>MDIKINDITLGNNSPFVLFGGINVLESLDSTLQTCAHYVEVTRKLGIPYIFKASFDKANRSSIHSYRGVGLEEGLKIFEKVKAEFGIPVITDVHEPHQCQPVAEVCDVIQLPARLAQQTDLVVAMAKTGNVVNIKKPQGLSPSQMKNIVEKFHEAGNGKLILCERGSSFGYDNLVVDMLGFGVMKQTC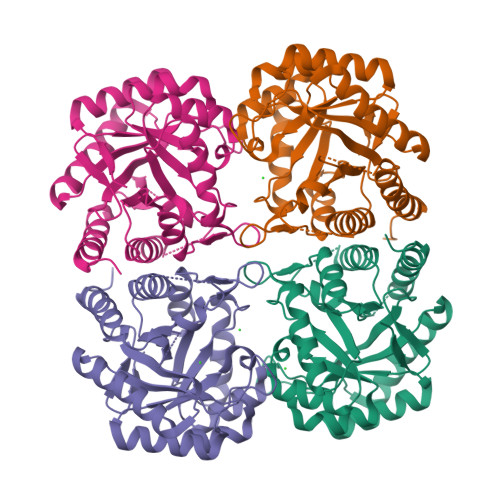GNLPVIFDVTHSLQTRDAGSAASGGRRAQALDLALAGMATRLAGLFLESHPDPKLAKCDGPSALPLHLLEDFLIRIKALDDLIKSQPILTIE[4x]> MSLHFLYYCSEPTLDVKIAFCQGFDKQVDVSYIAKHYNMSKSKVDNQFYSVEVGDSTFTVLKRYQNLKPIGSGAQGIVCAAYDAVLDRNVAIKKLSRPFQNQTHAKRAYRELVLMKCVNHKNIISLLNVFTPQKTLEEFQDVYLVMELMDANLCQVIQMELDHERMSYLLYQMLCGIKHLHSAGIIHRDLKPSNIVVKSDCTLKILDFGLARTAGTSFMMTPYVVTRYYRAPEVILGMGYKENVDIWSVGCIMGEMVRHKILFPGRDYIDQWNKVIEQLGTPCPEFMKKLQPTVRNYVENRPKYAGLTFPKLFPDSLFPADSEHNKLKASQARDLLSKMLVIDPAKRISVDDALQHPYINVWYDPAEVEAPPPQIYDKQLDEREH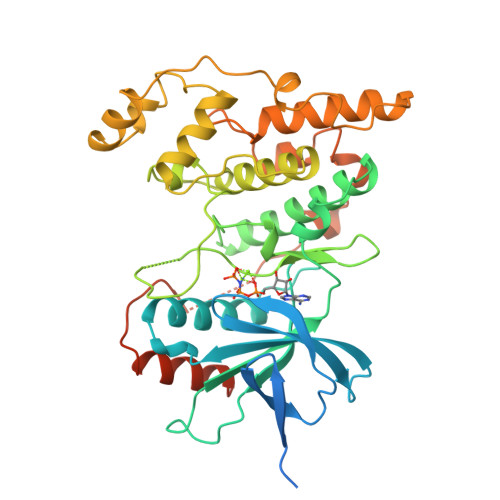TIEEWKELIYKEVMNSEEKTKNGVVKGQPSPSGAAVNS>QYVRIKNWGSGEILHDTLHHKATSDFTCKSKSCLGSIMNPKSLTRGPRDKPTPLEELLPHAIEFINQYYGSFKEAKIEEHLARLEAVTKEIETTGTYQLTLDELIFATKMAWRNAPRCIGRIQWSNLQVFDARNCSTAQEMFQHICRHILYATNNGNIRSAITVFPQRSDGKHDFRLWNSQLIRYAGYQMPDGTIRGDAATLEFTQLCIDLGWKPRYGRFDVLPLVLQADGQDPEVF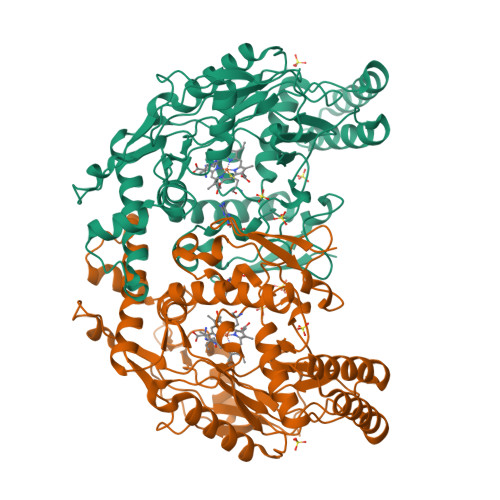EIPPDLVLEVTMEHPKYEWFQELGLKWYALPAVANMLLEVGGLEFPACPFNGWYMGTEIGVRDFCDTQRYNILEEVGRRMGLETHTLASLWKDRAVTEINVAVLHSFQKQNVTIMDHHTASESFMKHMQNEYRARGGCPADWIWLVPPVSGSITPVFHQEMLNYVLSPFYYYQIEPWKTHIWQ[2x]> MAQQDGPTPEPSVGSRTVLVYMIAQNSLAPLA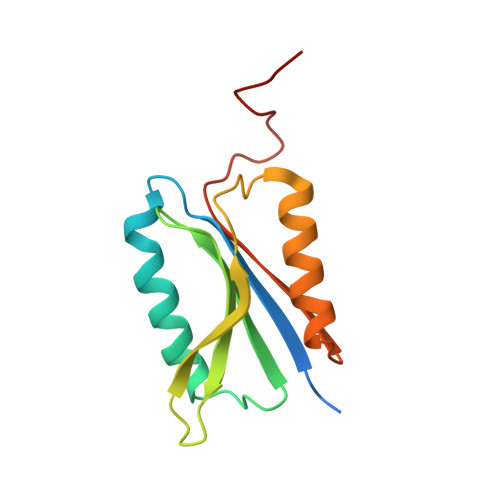SADIEEMKEGMRQVDATSGNLLVYIDDYSAPRLIRLGKDKKGKVVEETIENYPEQNSADANVMKKVISTAFNQYKAEKYGMVFWSHGEGWIPSPAKTR>[2x]SGTGSDDLKFVFVM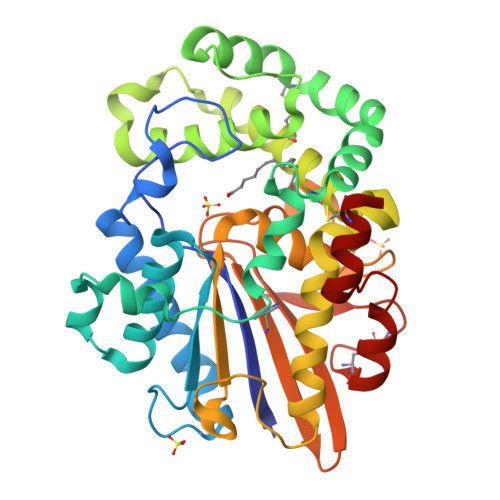ARGGDFVAGDYAGGPKIINKEAKDSELTEQGKQEAFQLGTKLSGLYKTKLGVSKWDSKTYWPVAISQKRAQVSTLITGAGLEGDQSKRDKTWTDQELKATSFPAMESFSRFIKPSECPNYLKELLAQQGEITTIVKECISSVQQVKSKYPAVDEKMPQHIWLAYETLKKLKRQQPSSSTWMTDDLMKNLRECSAKITWLATTKTDTLRKLSGGLLLNDLFNDMDQITQGKAQPNAPGGKDSKLNVFTVSQFLVISQLAAFMPEGSKLNNKAVTASDIYPEDGSHVDIEMYQENNKWSVKLVYVSGKDKQPQTITLPGCQEKCPYEQFKSALQKYKITDEEHQKACKN>GIDPFTMVVKKRKLATEAGGSDERPKYLPGKHPKNQEKTPHVDYNAPLNPKSELFLDDWHIPKFNRFISFTLDVLIDKYKDIFKDFIKLPSRKFHPQYYYKIQQPMSINEIKSRDYEYEDGPSNFLLDVELLTKNCQAYNEYDSLIVKNSMQVVMLIEFEVLKAKNLKRNYLINSEVKAKLLHYLNKLVDATEKKINQALLGASSPKNLDDKVKLSEPFMELVDKDELPEYYEIVHSPMALSIVKQNLEIGQYSKIYDFIIDMLLVFQNAHIFNDPSALIYKDATTLTNYFNYLIQKEFF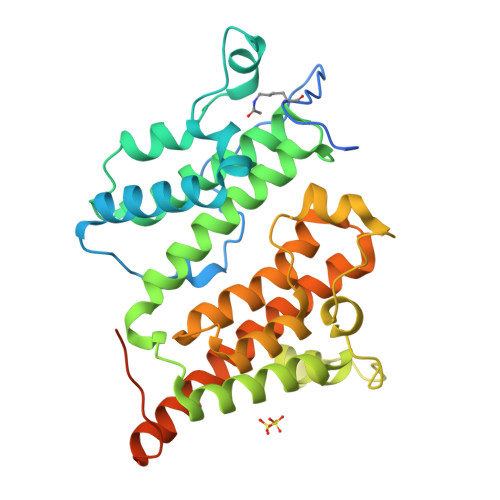PELQDLNERGEINLEFDKFEFENYLAIGGGGPAAAGALAISALDND[3x]>[12x]MKYVVVSGGVISGIGKGVLASSTGMLMKTLGLKVTSIKIDPYMNIDAGTMSPLEHGECFVLDDGGETDLDLGNYERYLGVTLTKDHNITTGKIYSHVIAKERKGDYLGKTVQIVPHLTNAIQDWIERVAKIPVDDTGMEPDVCIIELGGTVGDIESAPFVEALRQFQFKVGKENFALIHVSLVPVIHGEQKTKPTQAAIKGLRSLGLVPDMIACRCSETLDKPTIDKIAMFCHVGPEQVVNVHDVNSTYHVPLLLLEQKMIDYLHARLKLDEISLTEEEKQRGLELLSKWKATTGNFDESMETVKIALVGKYTNLKDSYLSVIKALEHSSMKCRRKLDIKWVEATDLEPEAQESNKTKFHEAWNMVSTADGILIPGGFGVRGTEGMVLAARWARENHIPFLGVCLGLQIATIEFTRSVLGRKDSHSAEFYPDIDEKNHVVVFMMRLGLRPTFFQNETEWSQIKKLYGDVSEVHERHRHRYEINPKMVDELENNGLIFVGKDDTGKRCEILELKNHPYYIATQYHPEYTSKVLDPSKPFLGLVAASAGILQDVIEGKYDLEA

CTP synthase (CTPS) catalyzes the final, rate-limiting step of de novo CTP biosynthesis (Lieberman, 1956). Each CTPS monomer consists of a glutaminase domain and an amido-ligase domain connected by an alpha helical linker. Glutamine hydrolysis in the glutaminase domain produces ammonia which is transferred through a channel into the amido-ligase domain, where it is ligated to UTP to form CTP in an ATP-dependent process. Budding yeast have two CTPS isoforms, Ura7 and Ura8, which share 78 % identical residues.

We solved filament structures of both Ura7 and Ura8 in substrate- (ATP and UTP) and product- (CTP) bound states. Ura7 filaments reached lower resolutions, 7.3 Å (substrates) and 3.7 Å (products), but the overall structures were indistinguishable from Ura8 at these resolutions. Because of their higher resolution which enabled building of atomic models, we focus subsequent structural interpretation on the Ura8 filaments. Like other previously reported structures of human, Drosophila, and E. coli CTPS, the yeast enzyme assembles as stacked tetramers. However, it does so using a completely different interaction interface, which was the same in both substrate- and product-bound yeast structures. Helix 356–370 in the glutaminase domain mediates interactions between tetramers, so that each protomer is involved in assembly contacts. His360 interacts with D370 which would be stabilized by protonation of His360 at low pH, and likely explains the pH-sensitivity of the assembly interaction. Residues painted similar (yellow) and different (red) from Ura8. In addition, Ura7 assembles with the W363/W392 hydrophobic core shown in Figure 3.>[2x]MSSPIDLESADEELEERGGIVGLLNRYRALIVAVLTVAVFCIAAYAIYDLTTEVRYDDVVHALTTTKISSVLLALLFTGLSFASLIFYDQNALEYIGKRLPFPHVALTSFSAYAVGNTAGFGALSAGAIRYRAYTRLGLSPDDITRVIAFVTLAFGLGLASVGAMALLVIADEIGPLISVDGLWLRLIAIAILAALAFVVYAGRNGREVRIGPVAVRLPDSRTWSRQFLVTAFDIAASASVLYVLLPETSIGWPGFFAIYAIAVGLGVLSHVPAGFGVFETIIIAWLGSSVNEDAVLSSLVLYRVIYNVIPLVIAIAAISVAELRR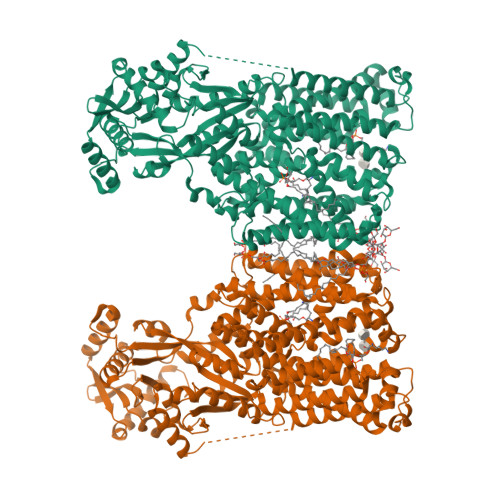FVDHPVASSMRRIGARLMPQLLSAFALLLGMMLVFSSVTPTPDHNLIVLSDYLPLSLVESAHFLSSLLGLAIIVAARGLSQRLDGAWWVSTFSALFALFFSLLKAIAIVEAGLLAFFVFSLVVSRRLFKRPASLLNQTLTAGWLTAIAVVCIGAIVVLFFVYRDVGYSNELWWQFEFADEAPRGLRAALGISIVSSAIAIFSLLRPATKRPEPVSDDAVARAVEIVRKQGVADANLVRMGDKSIMFSEKGDAFIMYGKQGRSWIALFDPVGPRQALPDLIWRFVETARAAGCRSVFYQISPALLSYCADAGLRAFKLGELAVVNLANFELKGGKWANLRQTASRAVRDGLEFAVIEPQDIPDVLDQLAHVSDTWLADHNAKEKSFSLGAFDPDYVCSQPVGVLKKDGKIVAFANILMTETKEEGSVDLMRFSPDAPKGSMDFLFVQILEYLKGEGFQRFNLGMAPLSGMSRRESAPVWDRVGGTVFEHGERFYNFKGLRAFKSKFHPEWQPRYLAVSGGVSPMIALMDATFLIGGGLKGVVRKKLAAALEHHHHHH> ETGSCAHMKQQVSFTGIQGDSARITCQVSNAVSYWIHWYRFQDGKPPQRLLCLSRESGELLFDEGFGSNKFHAFKDQFNGEKFILLIKKLEVRDSGMYYCAIWDWDGLVKVFGEGTRLIVTE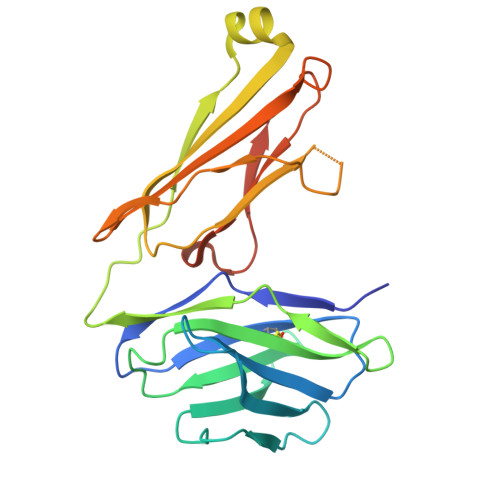SAFKKKPPKPIFFLPTSEEIKQKQSGTYICLLEDFFPNVVKTYWKEDGNSQPLDAQFGPITGGGNSYSQVSWLTVKEDVLRKNLTYFYQHEDLGMEPKAFSISSVREKGSLVPR>MPNLEPAVVVPTSEAIAVDLTKLEEKLAPADSFLDRHLGPGETEQRQMLQTLGFDTLGDLIDQAVPPAIRFPRSLQLPASQSEYGAIAQLKSIASKNQVFRSYIGMGYYDTITPPVIQRNILENPGWYTAYTPYQAEIAQGRLEALLNFQTMVMDLTGLEIANASLLDEGTAAAEAMALSYGVSKSKANAFFVAQDCHPQTIEVIKTRANPLGIEVIVGDHHTFSFSTSIFGALLQYPATDGAVYDYRSFIDKAHQHQALVTLAADPLSLTLLTPPGELGADIAVGSTQRFGIPLGYGGPHAAYFATKAEYQRKMPGRIVGVSKDAHGNPALRLALQTREQHIRRDKATSNICTAQVLLAVMASMYGVYHGSTGLKNIALRIHQLTVLLAIGLKRLNYSLNNDYFFDTLRVGVGEQSAPAILKAAEGRGINLRPLVPGEVGISLDETVTVQDLLDLWQVFAGKDNLPFTPEELWSEVKTSFPADLTRQSLYLQDAVFNQYHSETELLRYLHQLESKDLALNTSMIPLGSCTMKLNATAEMMPVTWPEFGKIHPFAPAGQTEGYQILFAQLEAWLGEITGFDAISLQPNAGSQGEYAGLQVIRQYHLSRGEEQRNICLIPESAHGTNPASAVMCGMQVVPVKCDGEGNIDVEDLTSKAEKYGDRLAALMVTYPSTHGVFEATIGTICDIVHRFGGEVYMDGANMNAQVGLCRPADFGADVCHLNLHKTFCIPHGGGGPGMGPIGVKSHLQAFLPRTSLNSTAELQAEDQSIGMISAAPYGSASILVISWMYIAMMGPQGLTKATEVAILSANYMAKRLENYYPILFRGNNELVAHECILDLRPLKKQAAIEVEDVAKRLMDFGFHAPTVSWPVLGTMMVEPTESESLGELDRFCDAMIAIYQEAQAITHGEIDPADNPLKNAPHTAQSLICGEWNHPYSQEEAAYPAPWTKQFKFWPAVGRINNTYGDRHLVCSCEGMEAYKE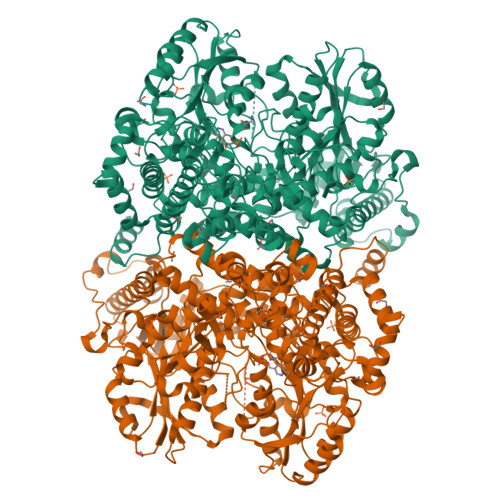G[2x]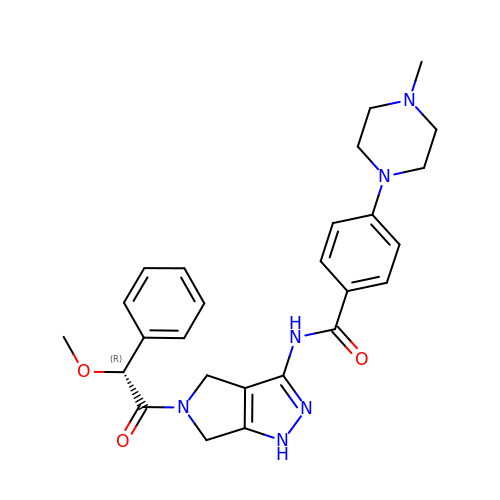N-[(3E)-5-[(2R)-2-METHOXY-2-PHENYLACETYL]PYRROLO[3,4-C]PYRAZOL-3(5H)-YLIDENE]-4-(4-METHYLPIPERAZIN-1-YL)BENZAMIDE | C26 H30 N6 O3 | XKFTZKGMDDZMJI-HSZRJFAPSA-N LRRK2 is a large multidomain protein with 2,527 amino acids (286 kDa) and consists of armadillo repeats (ARM), ankyrin repeats (ANK), leucine-rich repeats (LRR), Ras of complex (ROC), C-terminal of ROC (COR), kinase domain (KD), and the Trp-Asp-40 (WD40) domain. The C-terminal WD40 domain of LRRK2 is required for LRRK2-induced neurotoxicity and has been shown to mediate the interaction of LRRK2 with microtubules and synaptic vesicles. The structure reveals a canonical seven-bladed WD40 fold and a surprising dimeric state in the crystal. We found that the WD40 domain forms dynamic dimers in solution, and both structure-based mutations and PD-associated disease variants in the WD40 domain mainly impair its dimerization.

Here, we report the crystal structure of human LRRK2 WD40 domain determined at 2.6-Å resolution. We determined the WD40 domain crystal structure using the single wavelength anomalous diffraction (SAD) method and refined it to 2.6-Å resolution. The ordered part of the structure extends from residue 2,142 to residue 2,498 and has a few gaps, and the last 30 residues in the construct are disordered. The first six blades run from β2–β5, β6–β9, β10–β13, β14–β17, β18–β21, and β22–β25 continuously, and the last and seventh blade contains β26–β28 and β1 from the N-terminal end to complete the fold, forming a stabilized ring-like structure. There are two WD40 domain monomers in the crystallographic asymmetric unit, which are related by an almost perfect twofold axis (176.3°). The interactions are centered at blade V but also involve the surrounding structures as well as blade IV and VI. The dimerization interface is large and buries approximately ∼1,200 Å2 surface area per monomer. In addition to surface area burial, a number of potential hydrogen bonding and salt bridge interactions exist, among D2388 of one subunit and H2391 and S2345 of the symmetric subunit, among R2394 of one subunit and main chain atoms of M2408 and Y2410 of the symmetric subunit, and between E2395 of one subunit and Y2346 of the symmetric subunit. Notably, the WD40 domain mutation G2385R is located at the dimerization interface and compromised dimerization. Therefore, the WD40 domain dimer observed in the crystal is also a bona fide dimer in solution, instead of a crystallization artifact.

>GGSRRILLPKNVIVECMVATHHNSRNASIWLGCGHTDRGQLSFLDLNTEGYTSEEVADSRILCLALVHLPVEKESWIVSGTQSGTLLVINTEDGKKRHTLEKMTDSVTCLYCNSFSKQSKQKNFLLVGTADGKLAIFEDKTVKLKGAAPLKILNIGNVSTPLMCLSESTNSTERNVMWGGCGTKIFSFSNDFTIQKLIETRTSQLFSYAAFSDSNIITVVVDTALYIAKQNSPVVEVWDKKTEKLCGLIDCVHFLREVMVKENKESKHKMSYSGRVKTLCLQKNTALWIGTGGGHILLLDLSTRRLIRVIYNFCNSVRVMMTAQLGSLKNVMLVLGYNRKNTEGTQKQKEIQSCLTVWDINLPHEVQNLEKHIEVRKELAEKMRRTSVE[2x]>MGNLSYADLITRAIESSPDKRLTLSQIYEWMVRCVPYFKDKGDSNSSAGW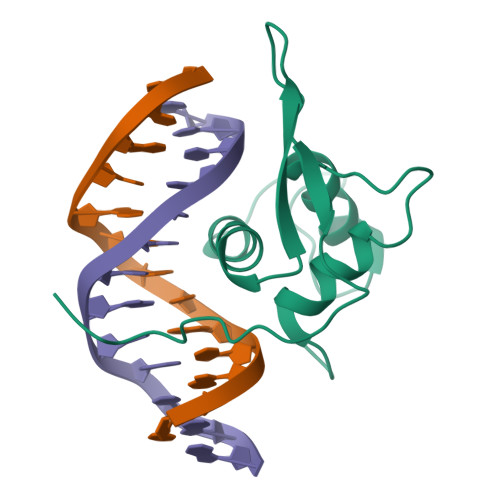KNSIRHNLSLHSRFMRVQNEGTGKSSWWIINPDGGKSGKAPRRRAVS[2x]(3E)-4-(2-HYDROXYPHENYL)-2-OXOBUT-3-ENOIC ACID | C10 H8 O4 | 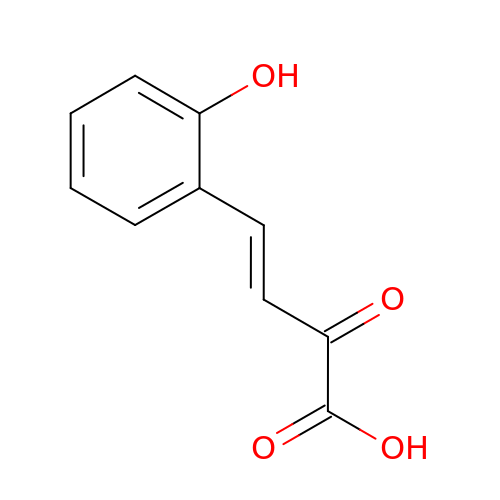HMXOGGUFCBUALL-UHFFFAOYSA-N> CDIHVLWEWECFEKL;>EVVKFMDVYQRSYCHPIETLVDIFQEYPDEIEYIFKPSCVPLMRCGGCCNDEGLECVPTEESNITMQIMRIKPHQGQHIG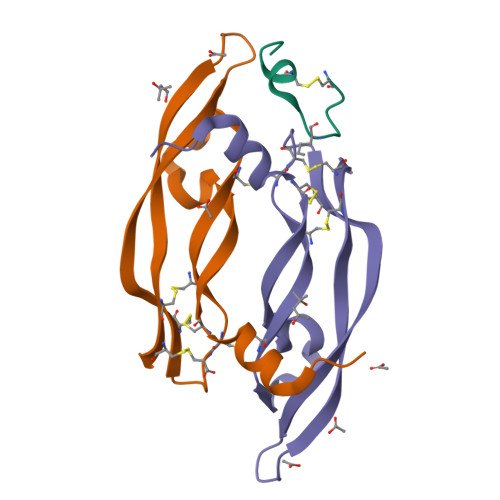EMSFLQHNKCECRPK[2x]(2S,4aR,6R,7R,7aS)-6-(6-amino-2-chloro-9H-purin-9-yl)-7-hydroxy-2-sulfanyltetrahydro-2H,4H-2lambda~5~-furo[3,2-d][1,3,2]dioxaphosphinin-2-one | C10 H11 Cl N5 O5 P S | 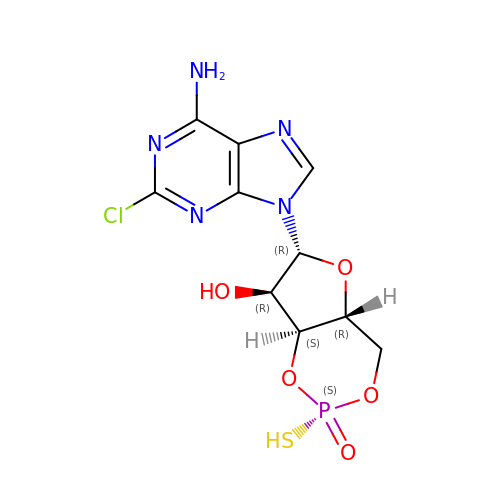PMTFGHJSNPKVBG-FHIGPPGSSA-N> AMPFEIEVLLPGELSPAETSALQKCEGKIITFSTLRHRASLVDIALSSYYINGAPPDTLSLLEAYRMRFAAVITRVIPGKLLAHAIGVGTPTPGLFIQNTSPVDLCNGDYICLLPPVYGSADSIRLDSVGLEIVFPLTIPQTLMREIIAKVVARAVEDLNLMFSINEGCLLILALIPRLLALLIPRLLALVT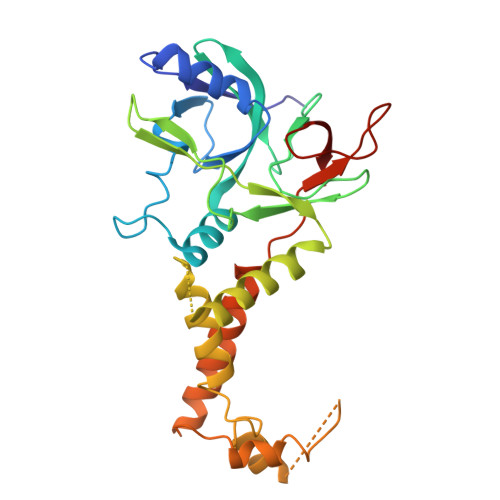REAAQLIHPEAPMLMLPIYETISSWISTSSRLGDTLGTRAILRVCVFDGPSTVHPGDRTAVIQV> MAWPKVQPEVNIGVVGHVAHGKTTLVQAITGIWTSKHSEELKRGMTIKLGYAETNIGVCESCKKPEAYVTEPSCKSCGSDDEPKFLRRISFIDAPGHEVLMATMLSGAALMDGAILVVAANEPFPQPQTREHFVALGIIGVKNLIIVQNKVDVVSKEEALSQYRQIKQFTKGTWAENVPIIPVSALHKINIDSLIEGIEEYIKTPYRDLSQKPVMLVIRSFDVNKPGTQFNELKGGVIGGSIIQGLFKVDQEIKVLPGLRVEKQGKVSYEPIFTKISSIRFGDEEFKEAKPGGLVAIGTYLDPSLTKADNLLGSIITLADAEVPV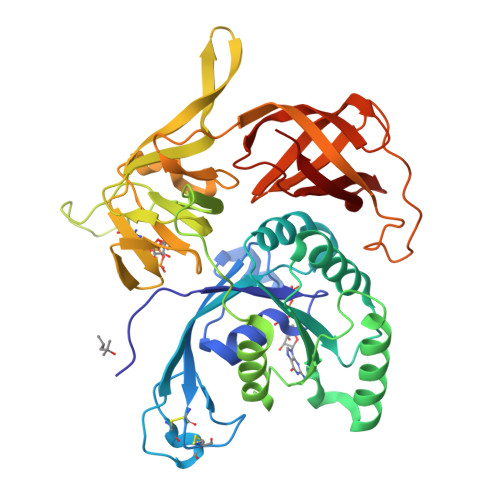LWNIRIKYNLLERVVGAKEMLKVDPIRAKETLMLSVGSSTTLGIVTSVKKDEIEVELRRPVAVWSNNIRTVISRQIAGRWRMIGWGLVEI>MITLKSAREIEAMDKAGDFLASIHIGLRDLIKPGVDMWEVEEYVRRRCKEENFLPLQIGVDGAMMDYPYATCCSLNDEVAHAFPRHYILKDGDLLKVDMVLGGPIAKSDLNVSKLNFNNVEQMKKYTQSYSGGLADSCWAYAVGTPSEEVKNLMDITKEAMYKGIEQAVVGNRIGDIGAAIQEYAESRGYGVVRDLVGHGVGPTMHEEPMVPNYGIAGRGLRLREGMVLTIEPMINTGDWEIDTDMKTGWAHKTIDGGLSCQYEHQFVITKDGPVILTSQGEEGTY[2x]

In about 60-70% of newly synthesized proteins, the initiator methionine is removed by a metalloenzyme called methionine aminopeptidase (MetAPs). Type Ia MetAP is the isoform with minimum sequence and structure required for the catalysis and is present in all prokaryotes. MetAPs have strict substrate specificity towards peptides with methionine on the amino-terminus. Here, we report the discovery of a novel MetAP1a found predominantly in the streptococci bacteria with two new structural motifs one of which may undergo posttranslational modification of glycosylation and phosphorylation.

To further understand the relationship of the two inserts with respect to catalytic domain, crystal structure of the SpMetAP1a is determined at 3.2 Å in the P65 space group with two molecules in the asymmetric unit. The overall structure is similar to that of the E. coli MetAP1a (EcMetAP1a) adopting the pita-bread fold. Since the crystals were grown in the absence of metal salts, the active site is devoid of any metal ions. The metal binding residues are well ordered and interact with each other as was noticed in the human MetAP1b apo structure. Although the overall structure of SpMetAP1a is similar to other MetAP structures in the catalytic domain, there is important difference near the active site. Not withstanding the confirmation of the extra loops (discussed below), a β-hairpin198-211 (equivalent region in EcMetAP1a is 170-183) undergoes a conformational change and occupies the active site where the substrate methionine usually binds. In the new conformation, the metal binding H199 moves away from the active site when compared to analogous residue (H171) in EcMetAP1a. Due to this flip of the β-hairpin, residues in the loop region are forced to occupy the substrate-binding region. Hence, substrate cannot bind to the enzyme in this conformation. The insert region (103Gly–Gly132) forms the extension of the loop within a beta-hairpin. The tyrosine kinase phosphorylation motif (124KKYT) is also well ordered and structurally placed closed to the glycosylation motif.> PLGSDGLPLDPRDWTRADVWKWLINMAVSEGLEVTA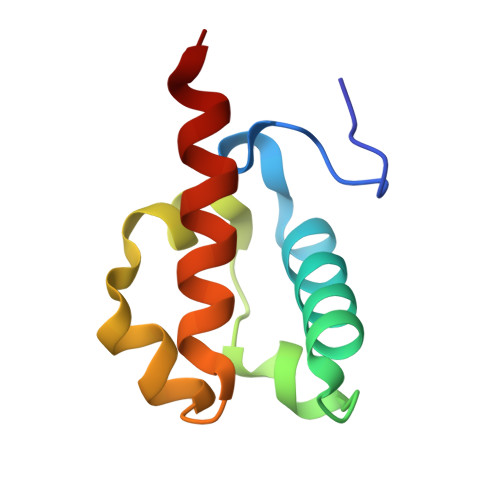ELPQKFPMNGKALCLMSLDMYLCRVPVGGKMLYRDFRVRLARAMSR The genus Enterovirus within the Picornaviridae, a family of non-enveloped viruses with a positive single-stranded RNA genome, is comprised of more than 100 serotypes. Human enteroviruses (EV) are presently classified into four groups, Enterovirus A-D (EV-A, B, C, and D), among which EV-B, the largest group, consists of over 60 serotypes, including all 6 serotypes of coxsackievirus B (CVB1-6), coxsackievirus A9 (CVA9), over 30 serotypes of echoviruses and more than 20 newly identified enteroviruses. The capsid proteins (VP1, VP2, and VP3) adopt the classical eight-stranded anti-parallel β-barrel configuration with the N-termini residing inside and the C-termini exposed on the surface. Most of the uncoating receptors bind to the “canyon” sites of the viral particle, dislodging the “pocket factor” in VP1 and subsequently triggering conformational changes of the intact particle to release the genome, albeit that SCARB2 binds EV71 outside the canyon.

We also determined the atomic structures of E30 in complex with its receptor FcRn and CD55. We determined the cryo-EM structures of E30 F-particle in complex with FcRn and CD55 under neutral conditions at 3.3 Å and 3.6 Å, respectively and obtained atomic models for these two complexes. Bindings of FcRn and CD55 have minimal impact on the capsid structure with RMSDs of 0.3 Å and 0.4 Å, respectively between mature and complexed viruses. However, in FcRn-bound viruses, the pocket factor was released and the pocket partially collapsed with the side chains of Tyr147, Asn215, and Met217 repositioning to decrease the pocket volume, similar to the pocket observed in E-particle, whilst there is no notable reduction in the amount of the pocket factor in CD55-bound viruses, indicative of that FcRn is capable of triggering viral pocket factor dislodgement, but CD55 might only facilitate viral attachment at neutral pH. Compared to FcRn, the interactions between E30 and CD55 are reduced by nearly half, where the short consensus repeat (SCR) 3 of CD55 contacts both VP1 GH and VP2 EF loops in E30 via hydrophilic interactions. In addition, CD55 presents a distinct attachment pattern to E30 in that the binding site lies outside the canyon, extending to the “south”. This site is roughly similar to those observed for SCARB2 binding to EV71 and for integrin binding to foot and mouth disease virus.

> NDPESALNRAVGRVADTVASGPVNTEQIPALTAVETGHTSQVVPSDTMQTRHVINYHTRSESSIENFMGRAACVYIAQYATEKVNDELDRYTNWEITTRQVAQLRRKLEMFTYMRFDLEITFVITSSQRTSTTYASDSPPLTHQVMYVPPGGPIPKSYEDFAWQTSTNPSVFWTEGNAPPRMSIPFMSVGNAYCNFYDGWSHFSQSGVYGYTTLNNMGHLYFRHVNKSTAYPVNSVARVYFKPKHVKAWVPRAPRLCPYLKARNVNFNVQGVTESRNKITLDRSTHNPLANT;> SPTVEECGYSDRVRSITLGNSTITTQECANVVVGYGVWPTYLSDHEATAVDQPTQPDVATCRFYTLESVKWESSSAGWWWKFPEALSDMGLFGQNMQYHYLGRTGYTIHVQCNASKFHQGCLLVVCVPEAEMGAATTDHAFNHTKLSNIGQAMEFSAKKSTDQTGPQTAVHNAGMGVAVGNLTIFPHQWINLRTNNSATIVMPYINSVPMDNMYRHYNFTLMVIPFAKLEHSPQASTYVPITVTVAPMCAEYNGLRLAGHQ;> GLPTMNTPGSTQFLTSDDFQSPSAMPQFDVTPEIQIPGQVRNLMEIAEVDSVVPVNNTEGHVNSMEAYRIPVRPQTSSGEQVFGFQLQPGHDSVLKHTLLGEILNYYANWSGSMKLTFMYCGAAMATGKFLIAYSPPGAGVPGSRRDAMLGTHVIWDVGLQSSCVLCVPWISQTNYRYVTSDAYTDAGYITCWYQTSIVTPPDIPTTSTILCFVSACNDFSVRLLRDTPFITQQALFQ;> GAQVSTQKTGAHETGLNASGNSIIHYTNINYYKDSASNSLNRQDFTQDPSKFTEPVKDVMIKTLPALN;> CNRSCEVPTRLNSASLKQPYITQNYFPVGTVVEYECRPGYRREPSLSPKLTCLQNLKWSTAVEFCKKKSCPNPGEIRNGQIDVPGGILFGATISFSCNTGYKLFGSTSSFCLISGSSVQWSDPLPECREIYCPAPPQIDNGIIQGERDHYGYRQSVTYACNKGFTMIGEHSIYCTVNNDEGEWSGPPPECRG N-(4-phenylbutyl)adenosine | C20 H25 N5 O4 | 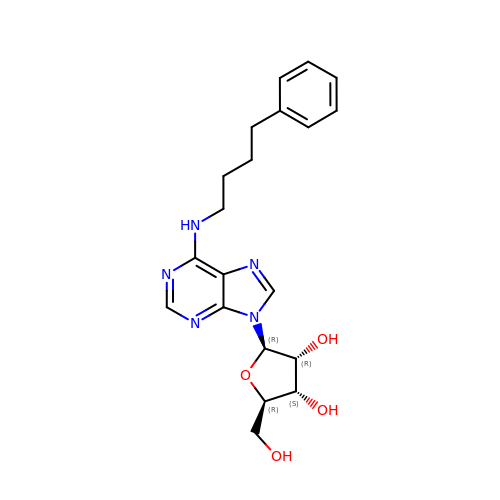QNQVVNSRYWTXJV-WVSUBDOOSA-N(2S,3S,11bS)-3-[3-(fluoromethyl)phenyl]-9,10-dimethoxy-1,3,4,6,7,11b-hexahydro-2H-pyrido[2,1-a]isoquinolin-2-amine 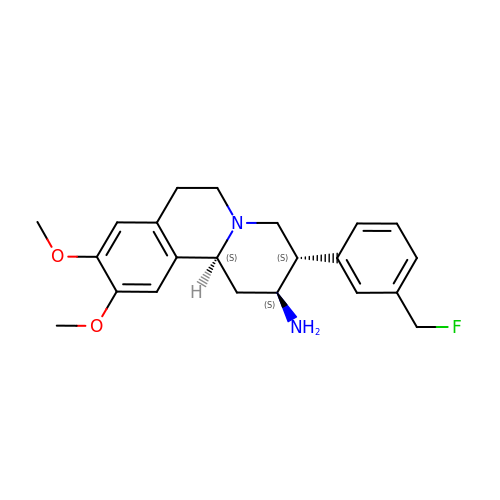| C22 H27 F N2 O2 | OQMKJZHTWPQABR-AABGKKOBSA-N> MRFRPFTEEDLDRLNRLAGKRPVSLGALRFFARTGHSFLAEEGEEPMGFALAQAVWQGEATTVLVTRMEGR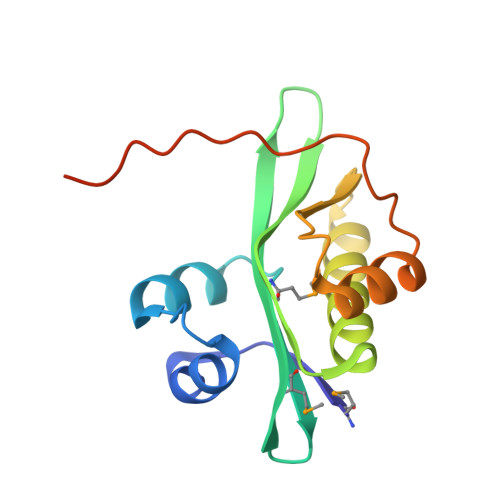SVEALRGLLRAVVKSAYDAGVYEVALHLDPERKELEEALKAEGFALGPLVLAVRVLGSRGARGETRGVLE>[2x]METLTVHAPSPSTNLP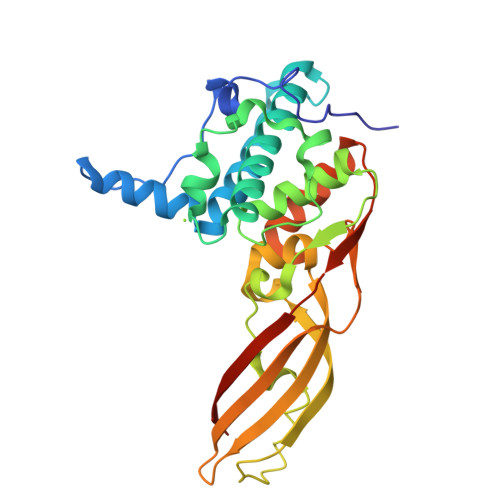SYGNGAFSLSAPHVPGAGPLLVQVVYSFFQSPNMCLQALTQLEDYIKKHGASNPLTLQIISTNIGYFCNADRNLVLHPGISVYDAYHFAKPAPSQYDYRSMNMKQMSGNVTTPIVALAHYLWGNGAERSVNIANIGLKISPMKINQIKDIIKSGVVGTFPVSTKFTHATGDYNVITGAYLGNITLKTEGTLTISANGSWTYNGVVRSYDDKYDFNASTHRGIIGESLTRLGAMFSGKEYQILLPGEIHIKESGKRAHHHHHH1H-INDAZOL-6-OL | C7 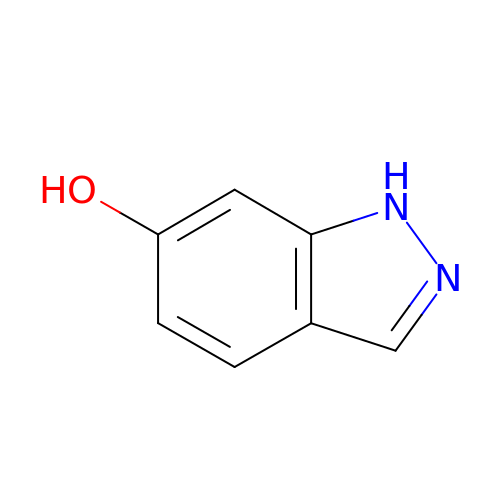H6 N2 O | NUYZVDBIVNOTSC-UHFFFAOYSA-N> MKNCVIVSAVRTAIGSFNGSLASTSAIDLGATVIKAAIERAKIDSQHV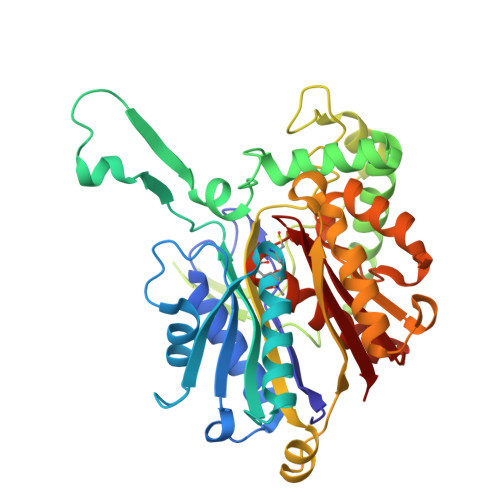DEVIMGNVLQAGLGQNPARQALLKSGLAETVCGFTVNKVCGSGLKSVALAAQAIQAGQAQSIVAGGMENMSLAPYLLDAKARSGYRLGDGQVYDVILRDGLMCATHGYHMGITAENVAKEYGITREMQDELALHSQRKAAAAIESGAFTAEIVPVNVVTRKKTFVFSQDEFPKANSTAEALGALRPAFDKAGTVTAGNASGINDGAAALVIMEESAALAAGLTPLARIKSYASGGVPPALMGMGPVPATQKALQLAGLQLADIDLIEANEAFAAQFLAVGKNLGFDSEKVNVNGGAIALGHPIGASGARILVTLLHAMQARDKTLGLATLCIGGGQGIAMVIERL> EFHMEMIRPSIQTILQDILSFSGLNPGRSSKRYRGFKSLLSRIIANDKKCRYDILYAKFIGTSKCNFANVVSNKTEISQVIQFVLLVLGKLLPLDAWGGVSNKKIIKDRVVDFLLLGANEKIHMDDLFRGIRLKDFKWLGRAHQISSKQDFELRTAFLKGYLWWLFEHLLKNILRSFWYITETSSIVSLELNYFPQYLWKELYESWVSKYAKNNLVKMPSKIQREQLPCGKIKLIPKRSSFRVICVPIKRSLKLLNKKLELDTLEKEKREFERYRKEVLSPVGQILRLKLSKLRDTYESYRASVHSSSDVAEKISDYRDSLLTRFGEIPKLFILKFDMKECYDRLSQPVLMKKLEELFENQDNKTSYYVRYYAQLDASHKLKKVKTTIDTQYHNLNILSSSRHLSNCKSLVDKTKTIALQKGNILEVCRSQI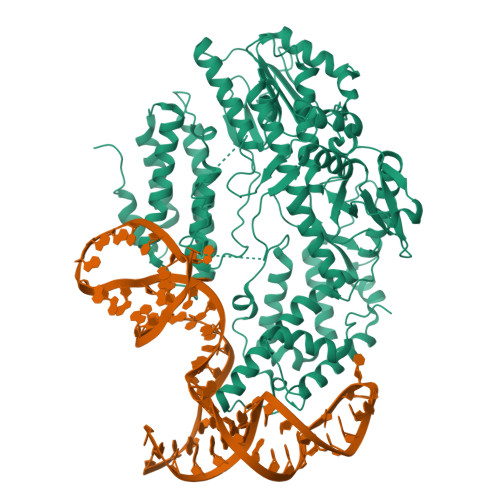YDVVGSVKDARGNLHLYKRKRGVFQGFSLSSIFCDILYSAMVHDCFQFLWKSKQDFLFVRLVDDFLLVTPDSNIYDQVHNILSGKILESYGAFVNKDKTVVVNQTTTKPSIDFVGLEVNTTDLSIKRNSGSISLVTTNFRTFKTLVKYLKTFYQLNLEGFLLDCSFGVLENVLENMGSLLRLVLREFKTKFTSIVKYDTFHCYKFIKFLYDISNYTIVKYVETNSDWDGAPELLNCIKQIIVKEFSSFESYSEIVEWVQTLNIVD(2R,3R)-N,2,3,4-TETRAHYDROXYBUTANAMIDE | C4 H9 N O5 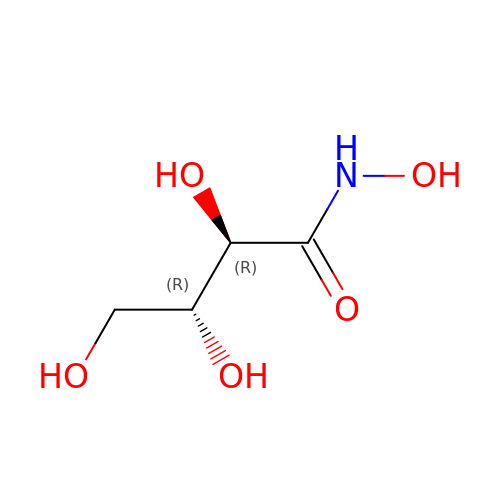| SJYJPXDRLWCEKB-PWNYCUMCSA-N> MAASSSGEKEKERLGGGLGVAGGNSTRERLLSALEDLEVLSRELIEMLAISRNQKLLQAGEENQVLELLIHRDGEFQELMKLALNQGKIHHEMQVLEKEVEKRDSDIQQLQKQLKEAEQILATAVYQAKEKLKSIEKARKGAISSEEIIKYAHRISASNAVCAPLTWVPGDPRRPYPTDLEMRSGLLGQMNNPSTNGVNGHLPGDALAAGRLPDVLAPQYPWQSNDMSMNMLPPNHSSDFLLEPPGHNKENEDDV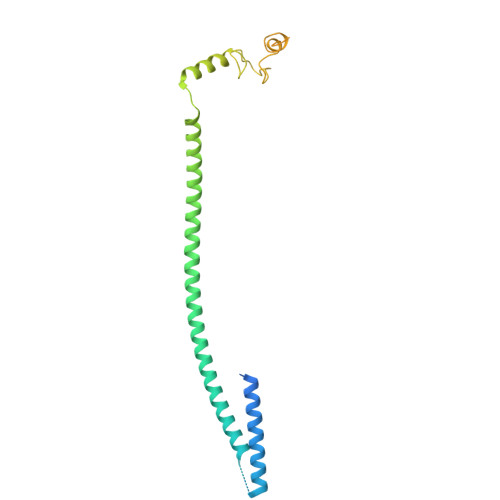EIMSTDSSSSSSESD> HMTPPKAEKRPYPITTHGDTRVDDYYWLRDDERTDPQVLDYLQAENAFTDAALKPQQALRETLYEEMVARIPQQEHSVPYVRHGYRYQTRFEPGNEYAIYVRQPQAESEHWDTLIDGNQRAEQREFYTLGGLEVSPDNQKLAVAEDFLSRRQYDIRFKNLSDDSWTDEVLENTSGSFEWANDSATVYYVRKHAKTLLPYQVYRHVVGTDPQLDELIYEEQDDTFYVGLEKTTSDRFILIHLSSTTTSEILLLDADRADSTPQMFVPRRKDHEYGIDHYHQHFYIRSNKDGKNFGLYQSEQADEAQWQTLIAPRIEVMLEGFSLFRDWLVVEERSEGLTQLRQIHWQSGEVKRIAFDDPTYTTWLAYNPEPETELLRYGYSSMTTPTTLYELNLDSDERVMLKQQEVKNFTPENYRSERVWVKARDGVEVPVSLVYRHDSFARGTNPLMVYGYGSYGSSMDPAFSASRLSLLDRGFVFVLAHIRGGGELGQLWYEDGKLFKKQNTFNDFIDVTEALIAQGYGDAKRVFAMGGAAGGLLMGAVINQAPELFNGIVAQVPFVDVVTTMLDESIPLTTGEYDEWGNPNQQAYYDYILQYSPYDQVKAQDYPHMLVTTGLHDSQVQYWEP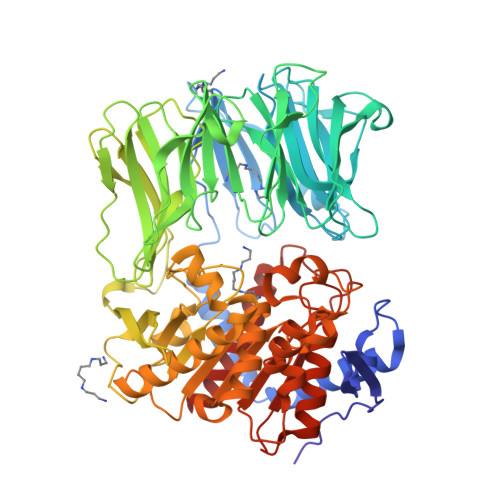AKWVAKLRELKTDDRQLLLYTDMDSGHGGKSGRFKAYEDIALEYAFILALAE> VYSYTEKKRIRKDFGKRPQVLDVPYLLSIQLDSFQKFIEQDPEGQYGLEAAFRSVFPIQSYSGNSELQYVSYRLGEPVFDVQECQIRGVTYSAPLRVKLRLVIYEREAPEGTVKDIKEQEVYMGEIPLMTDNGTFVINGTERVIVSQLHRSPGVFFDSDKGKTHSSGKVLYNARI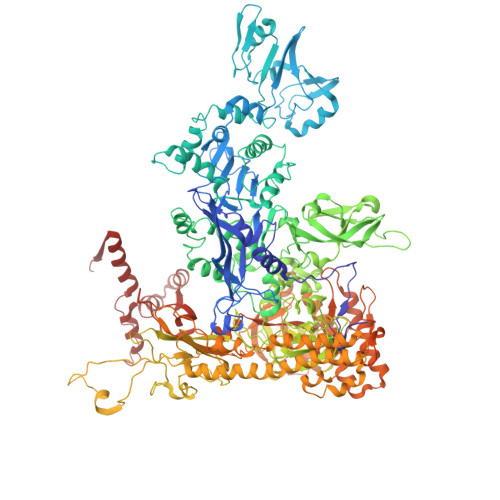IPYRGSWLDFEFDPKDNLFVRIDRRRKLPATIILRALNYTTEQILDLFFEKVIFEIRDNKLQMELVPERLRGETASFDIEANGKVYVEKGRRITARHIRQLEKDDVKLIEVPVEYIAGKVVAKDYIDESTGELICAANMELSLDLLAKLSQSGHKRIETLFTNDLDHGPYISETLRVDPTNDRLSALVEIYRMMRPGEPPTREAAESLFENLFFSEDRYDLSAVGRMKFNRSLLREEIEGSGILSKDDIIDVMKKLIDIRNGKGEVDDIDHLGNRRIRSVGEMAENQFRVGLVRVERAVKERLSLGDLDTLMPQDMINAKPISAAVKEFFGSSQLSQFMDQNNPLSEITHKRRISALGPGGLTRERAGFEVRDVHPTHYGRVCPIETPEGPNIGLINSLSVYAQTNEYGFLETPYRKVTDGVVTDEIHYLSAIEEGNYVIAQANSNLDEEGHFVEDLVTCRSKGESSLFSRDQVDYMDVSTQQVVSVGASLIPFLEHDDANRALMGANMQRQAVPTLRADKPLVGTGMERAVAVDSGVTAVAKRGGVVQYVDASRIVIKVNEDEMYPGEAGIDIYNLTKYTRSNQNTCINQMPCVSLGEPVERGDVLADGPSTDLGELALGQNMRVAFMPWNGYNFEDSILVSERVVQEDRFTTIHIQELACVSRDTKLGPEEITADIPNVGEAALSKLDESGIVYIGAEVTGGDILVGKVTPKGETQLTPEEKLLRAIFGEKASDVKDSSLRVPNGVSGTVIDVQVFTRDGVEKDKRALEIEEMQLKQAKKDLSEELQILEAGLFSRIRAVLVAGGVEAEKLDKLPRDRWLELGLTDEEKQNQLEQLAEQYDELKHEFEKKLEAKRRKITQGDDLAPGVLKIVKVYLAVKRRIQPGDKMAGRHGNKGVISKINPIEDMPYDENGTPVDIVLNPLGVPSRMNIGQILETHLGMAAKGIGDKINAMLKQQQEVAKLREFIQRAYDLGADVRQKVDLSTFSDEEVMRLAENLRKGMPIATPVFDGAKEAEIKELLKLGDLPTSGQIRLYDGRTGEQFERPVTVGYMYMLKLNHLVDDKMHARSTGSYSLVTQQPLGGKAQFGGQRFGEMEVWALEAYGAAYTLQEMLTVKSDDVNGRTKMYKNIVDGNHQMEPGMPESFNVLLKEIRSLGINIELEDE>ACDYTCGSACYSSSDVSTA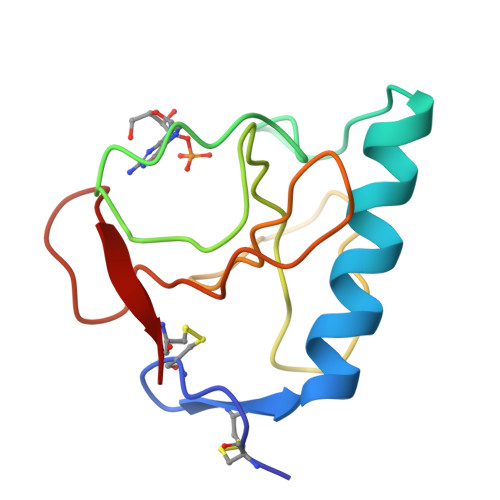QAAGYKLHEDGETVGSNSYPHKYNNYEGFDFSVSSPYYEWPILSSGDVYSGGSPGADRVVFNENNQLAGVITHTGASGNNFVECT[4x]>DFWCSTLVKGVIYGSYSVSEMFPKNFTNCTWTLENPDPTKYSIYLKFSKKDLSCSNFSLLAYQFDHFSHEKIKDLLRKNHSIMQLCSSKNAFVFLQYDKNFIQIRRVFPTDFPGLQKKVEEDQKSFFEFLVLNKVSPSQFGCHVLCTWLESCLKSENGRTESCGIMYTKCTCPQHLGEWGIDDQSLVLLNNVVLPLNEQTEGCLTQELQTTQVCNLTREAKRPPKEEFGMMGDHTIKSQRPRSVHEKRVPQEQADAAKFMAQTGAAALEVLFQ[3x];>[3x]DASHHHHHHSTVPKIAFYAGLKRQHEGYEVLKFDDVVTNLGNHYDPTTGKFTCSIPGIYFFTYHVLMRGGDGTSMWADLCKNNQVRASAIAQDADQNYDYASNSVVLHLEPGDEVYIKLDGGKAHGGNNNKYSTFSGFIIYAD

The adhesion-GPCR Brain-specific Angiogenesis Inhibitor-3 (BAI3) plays a crucial role in organizing synapses in the brain. BAIs are a family of adhesion-GPCRs comprising BAI1, BAI2 and BAI3 that are implicated in multiple developmental functions. However, how BAI3 engages one of its ligands, the C1q-like proteins (C1qls), remains largely unexplored. C1qls are thought to form large 18-meric assemblies, suggesting a higher oligomeric state of the complex and a potentially different interaction mode.

We then determined the structure of the mouse C1ql3-BAI3 NTD complex by single-particle cryoEM to a resolution of 2.8 Å. At the core of the complex, three globular C1q-like domains form a trimeric quaternary structure with four Ca2+-ions bound at the trimeric symmetry axis consistent with structures of the isolated C1q-like domain11. Three BAI3 NTDs bind to the C1ql3 trimer. Each BAI3 NTD interacts with the C1ql3 trimer at a composite interface between two C1ql3 molecules, creating a heterohexamer. Within the C1ql3-BAI3 interface, one C1ql3 copy establishes a Ca2+-mediated interaction with the BAI3 NTD. Asp180 and Asp232 of the C1q-like domain direct the coordination of the Ca2+-ion, while Lys66 and Asp63 of the BAI3 NTD participate in the water-mediated coordination of the Ca2+-ion. Furthermore, C1ql3 Trp188, BAI3 Lys66, and BAI3 Tyr67 engage in a π-stacking interaction that further stabilizes the complex. The second C1q-like domain in the binding interface also forms extensive interactions with the BAI3 NTD, where C1ql3 Tyr244 and Asn242 engage in hydrogen bonds with BAI3 Asp63, while C1ql3 Asn240 forms a hydrogen bond with BAI3 Glu60. In summary, each BAI3 molecule forms a Ca2+-mediated interface with the C1q-like domains of C1ql3 that is characterized by extensive intermolecular interactions and spans a total of ~564 Å2. Superposition of the BAI3 NTD onto the C1r CUB domain highlights a conserved core of β strands, with the primary distinction being that the BAI3 NTD contains additional α helices outside the core β sheet that are not usually present in CUB domains and that may mediate additional, as yet unidentified interactions by the NTD. In contrast, the trimeric C1q-like domains of C1ql3 bind to three copies of BAI3 in a 3:3 stoichiometry.>[6x]HHHHHHMEEEAETEEQQRFSYQQRLKAAVHYTVGCLCEEVALDKEMQFSKQTIAAISELTFRQCENFAKDLEMFARHAKRTTINTEDVKLLARRSNSLLKYITDKSEEIAQINLERKAQK;>GSIFSYRDGMRQSSLKKDWFLSEEEFKLWNRLYRLRDSDEI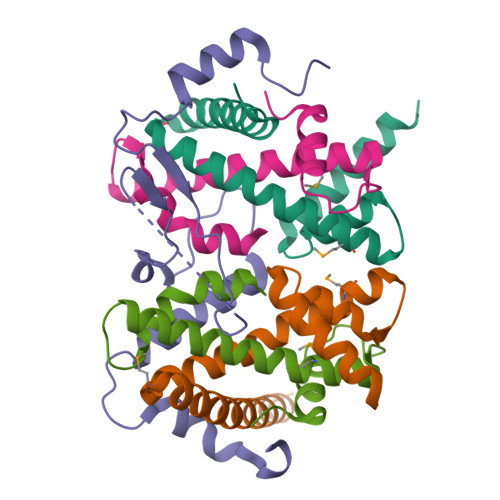KEITLPQVQFSSLQNEENKPAQESTTGIHQLSLSEWRLWQDHPLPTHQVDHSDRCRHFIGLMQMIEGMRHEEGECSYELEVESYLQMEDVTSTFIAPRNE[3x];>[6x]GSHMEGAGAGSGFRKELVSRLLHLHFKDDKTKVSGDALQLMVELLKVFVVEAAVRGVRQAQAEDALRVDVDQLEKVLPQLLLDF> YFTYDPYSEEDP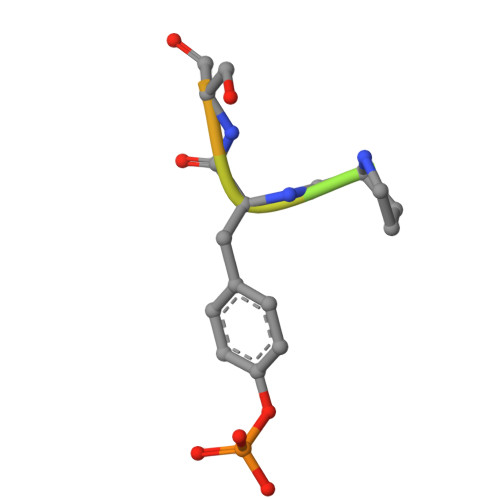D~{tert}-butyl (2'~{R},3~{R})-2'-[3-[4-(hydroxymethyl)-3-methylsulfonyl-phenyl]phenyl]-2-oxidanylidene-spiro[1~{H}-indole-3,3'-pyrrolidine]-1'-carboxylate | C30 H32 N2 O6 S | 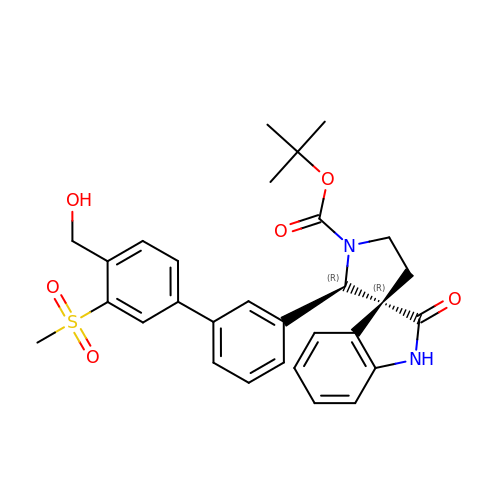WCOXMLFEWOILDZ-PDDLMNHVSA-N>GSSSPLPKVAHNLGFYFSPDLTQFAKLPAELAPHWPVVTTQNNERWPDRLVASLRPIHKYSRACIGAGYMVGPSVFLGTPGVVSYYLTKFVRGEAQVLPETVFSTGRIEVDCREYLDDRERVVAESLPHAFIGDVKGTTVGGCHHVTSKYLPRFLPKESVAVVGVSSPGKAAKAV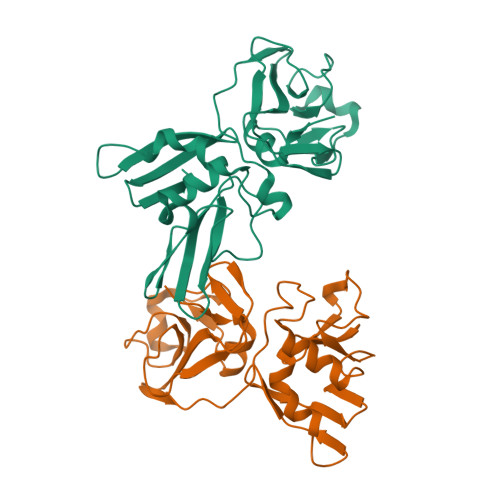CTLTDVYLPDLEAYLHPETQSRCWKVMLDFKEVRLMVWKDKTAYFQLEHHHHHH[2x]GLUCOSE-6-PHOSPHATE | C6 H13 O9 P | 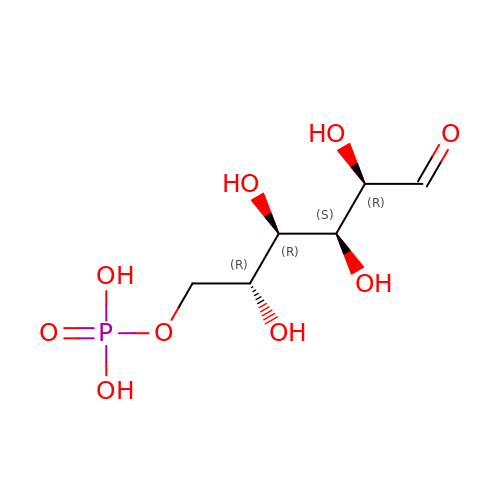VFRROHXSMXFLSN-SLPGGIOYSA-N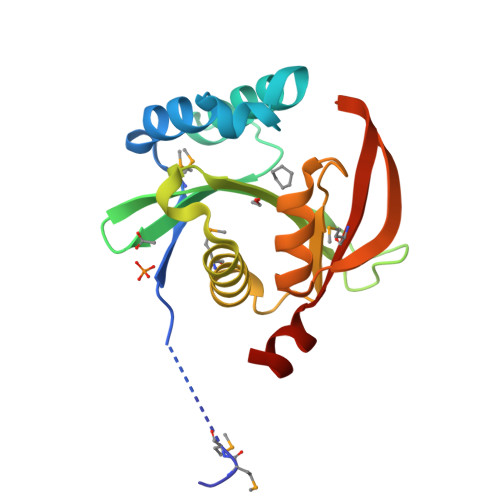> SNAMMIKASTNEFRFCFKQMNKSQHELVLGWIHQPHINEWLHGDGLSNTIKDLHEFLNDGKPWATHWIAYDNEIPFAYLITSEIEKSEEYPDGAVTLDLFICRLDYIGKGLSVQMIHEFILSQFSDTKIVLINPEISNERAVHVYKKAGFEIIGEFIASWHPVPHYKMKLCIEDLKKQRLSA>MTAPRSWAPTTRARGDTEALCSPEDGWVKVHPTPGTMLFREILHGQLGYTEGQGVYNVVRSSEATTRQLQAAIFHALLNATTYRDLEADWLGHVAARGLQPQRLVRRYRNAREADIAGVAERVFDTWRNTLRTTLLDFAHGLVACFAPGGPSGPSSFPKYIDWLTCLGLVPILRKRQEGGVTQGLRAFLKQHPLTRQLATVAEAAERAGPGFFELALAFDSTRVADYDRVYIYYNHRRGDWLVRDPISGQRGECLVLWPPLWTGDRLVFDSPVQRLFPEIV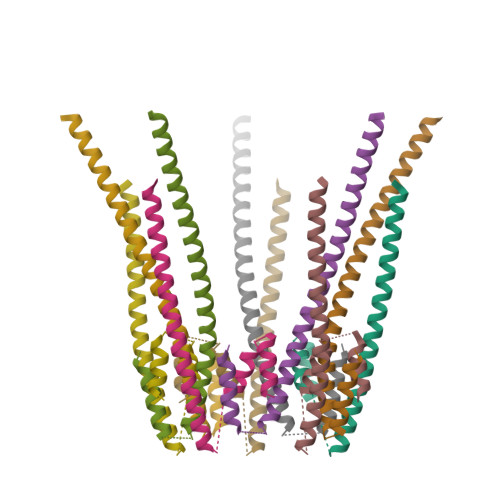ACHSLREHAHVCRLRNTASVKVLLGRKSDSERGVAGAARVVNKVLGEDDETKAGSAASRLVRLIINMKGMRHVGDINDTVRSYLDEAGGHLIDAPAVDGTLPGFGKGGNSRGSAGQDQGGRAPQLRQAFRTAVVNNINGVLEGYINNLFGTIERLRETNAGLATQLQERDRELRRATAGALERQQRAADLAAESVTGGCGSRPAGADLLRADYDIIDVSKSMDDDTYVANSFQHPYIPSYAQDLERLSRLWEHELVRCFKILCHRNNQGQETSISYSSGAIAAFVAPYFESVLRAPRVGAPITGSDVILGEEELWDAVFKKTRLQTYLTDIAALFVADVQHAALPPPPSPVGADFRPGASPRGRSRSRSPGRTAPGAPDQGGGIGHRDGRRDGRR[10x]> UG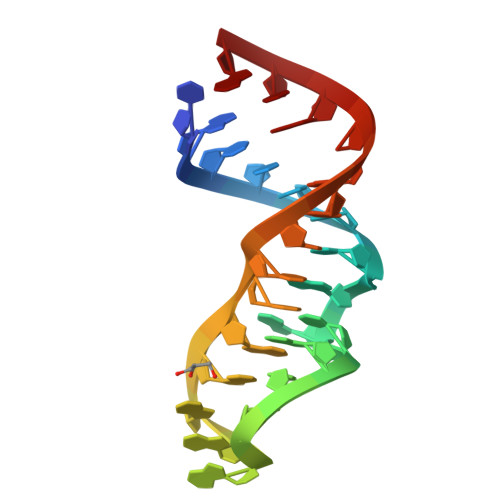CUCCUAGUACGAGAGGACCGGXGUG>GPHMLDLFADAEPWQEPLAAGAVILRRFAFNAAEQLIRDINDVASQSPFRQMVTPGGYTMSVAMTNCGHLGWTTHRQGYLYSPIDPQTNKPWPAMPQSFHNLCQRAATAAGYPDFQPDACLINRYAPGAKLSLHQDKAEPDLRAPIVSVSLGLPAIF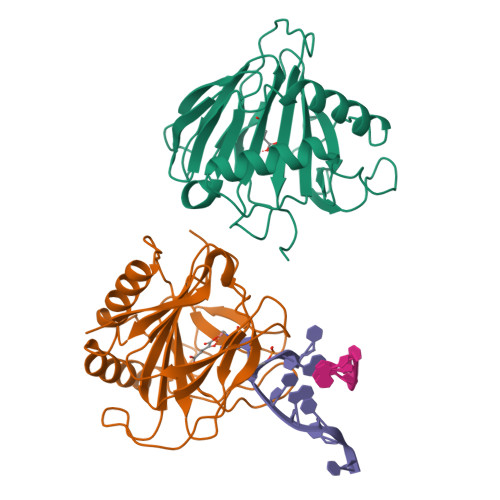QFGGLKRNDPLKRLLLEHGDVVVWGGESRLFYHGIQPLKAGFHPLTIDCRYNLTFRQAGKKE[2x]> SASPHYQEWIL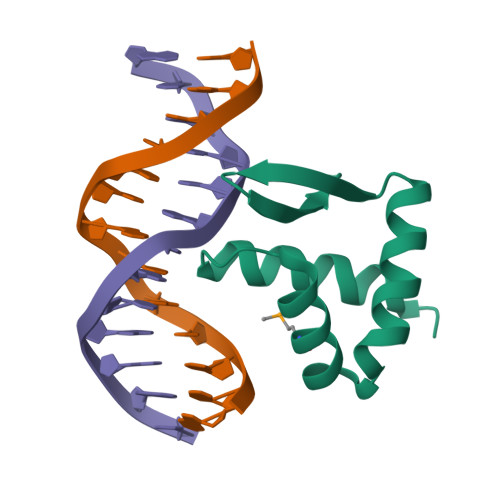DTIDSLRSRKARPDLERICRMVRRRHGPEPERTRAELEKLIQQRAVLRVSYKGSISYRNAARVQPPRRG The ESX-1 type VII secretion system is an important determinant of virulence in pathogenic mycobacteria, including Mycobacterium tuberculosis. This complicated molecular machine secretes folded proteins through the mycobacterial cell envelope to subvert the host immune response. All ESX gene clusters contain at least three or four ESX conserved components (Ecc), named EccB, EccC, and EccD, with EccE being present in all ESX systems with the exception of ESX-4. In this study we report the molecular structures of the periplasmic domain of EccB1 and the cytoplasmic domain of EccD1 from the ESX-1 cluster.

M. tuberculosis EccB1 (Rv3869) is a 51 kDa protein containing a 40 amino acid (aa) N-terminal domain followed by a single membrane-spanning helix and a ~400 aa C-terminal fold. In order to gain further insight into the role of EccB1 within the ESX machinery we determined the crystal structure of the C-terminal domains of EccB1 from M. tuberculosis (EccB1mt) to 1.7 Å resolution and of the orthologous protein (MSMEG_0060; EccB1ms) from the nonpathogenic mycobacterial species M. smegmatis to 3.07 Å resolution. Both EccB1 structures contain a single elongated fold in the shape of a distorted propeller, which has an unanticipated quasi 2-fold symmetry. The central core domain consists of a 6 stranded β-sheet with 5 strands (β7-β19-β18-β5-β6) arranged in anti-parallel fashion with an additional strand (β21) parallel to strand β6 on the periphery of the sheet; the sheet is further stabilized by a disulfide bond between the two central strands (β5 and β18) of the sheet formed between Cys150 and Cys345 (EccB1mt) and Cys152 and Cys347 (EccB1ms). The four repeat domains each contain a 4 stranded β sheet and two α helices. Repeat 1 (R1) (residues S74-M124) and repeat 4 (R4) (residues G391-L445) are located between the core domain and the N-terminal transmembrane region while repeat 2 (R2) (residues E185-P241) and repeat 3 (R3) (residues V267-A320) are located on the opposite side of the core domain distal to the transmembrane region. The interfaces between R1/R4 and R2/R3 domains are formed by hydrophobic residues on the N-terminal helices of each repeat that fold together with each other and with hydrophobic residues from the proline rich strands downstream of each repeat’s C-terminal helix. The R2 and R3 domains also pack tightly with the core domain via residues on their N-terminal helices as well as β sheet residues. Pairwise sequence alignments of the repeats shows that R2, R3, and R4 show 26, 33 and 27 % sequence identity, respectively, to R1. The elongated shape and continuous hydrophobic core of EccB1 suggest that it may serve a structural role – perhaps forming part of a structure that spans the inner and outer membrane components of the ESX secretion system.

> GAMGTSLFTDRATNQLYVLLSGQLHPVYNLTSARLVLGNPANPATVKSSELSKLPMGQTVGIPGAPYATPVSAGSTSIWTLCDTVARADSTSPVVQTAVIAMPLEIDASIDPLQSHEAVLVSYQGETWIVTTKGRHAIDLTDRALTSSMGIPVTARPTPISEGMFNALPDMGPWQLPPIPAAGAPNSLGLPDDLVIGSVFQIHTDKGPQYYVVLPDGIAQVNATTAAALRATQAHGLVAPPAMVPSLVVRIAERVYPSPLPDEPLKIVSRPQDPALCWSWQRSAGDQSPQSTVLSGRHLPISPSAMNMGIKQIHGTATVYLDGGKFVALQSPDPRYTESMYYIDPQGVRYGVPNAETAKSLGLSSPQNAPWEIVRLLVDGPVLSKDAALLEHDTL>[3x]MSRFDSGLPSVRQV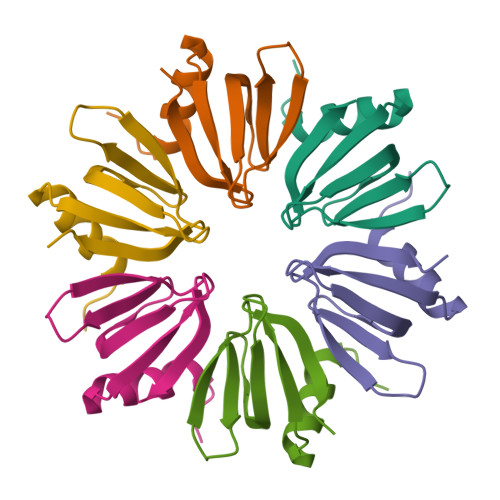QLLIKDQTPVEIKLLTGDSLFGTIRWQDTDGLGLVDDSERSTIVRLAAIAYITPRR>METESGNQEKVMEEESTEKKKEVEKKKRSRVKQVLADIAKQVDFWFGDANLHKDRFLREQIEKSRDGYVDISLLVSFNKMKKLTTDGKLIARALRSSAVVELDLEGTRIRRKKPLGERPKDEDERTVYVELLPKNVNHSWIERVFGKCGNVVYISIPHYKSTGDPKGFAFVEFETKEQAAKAIEFLNNPPEEAPRKPGIFPKTVKNKP[2x]

LARP7 is the family member showing the highest sequence similarity to La, with the characteristic La module in the N-terminal third of the protein. However, while La binds all nascent transcripts synthesized by RNA polymerase III via their shared termination motif, UUUOH, LARP7 binds almost exclusively to the non-coding RNA 7SK. The 7SK-specific 5′ cap is mono-methylated at the gamma phosphate of the 5′ triphosphate by another component of the 7SKsnRNP, MePCE (also called BCDIN3 in Drosophila). Together, MePCE and LARP7 bind 7SK on both ends, thus forming a stable 7SKsnRNP core protecting the RNA from exonucleases. Following a short unfolded region containing positively charged amino acids (1–27), the La module comprises two structured domains, one containing the LAM (residues 28–111) and the second, an RNA-recognition motif (RRM1; residues 120–199) according to a global analysis of the LARP superfamily.

The crystal structure of the LARP7 N-terminal domain, described here, is the first 3D structure of the La module of a member of the LARP family different from La showing the linked domains of the La module in a complex with RNA. The structure was solved from a crystal obtained in a drop initially set up with the hairpin HP4 (300–332). Indeed, difference Fourier showed densities for only three and five nucleotides in monomers A and B, respectively. The triplet of uridines at the 3′-end of 7SK binds into the cleft between the LAM and RRM1 domains. It is constrained in a characteristic hooked conformation, allowing strict recognition of the penultimate uridine, with a contribution of the RRM1 revealing LARP7 specificity. As was observed in La protein, the penultimate U-2 (numbering as in La) is anchored at the bottom of the crevice, and U-1 (the 3′-terminal uridine) at the surface of the LAM domain. The uridine U-3 stacks on U-1, leading to a characteristic fishhook shape of the backbone. The base ring is sandwiched between Phe44 from LAM and His138 from RRM1, in a pocket closed by Tyr153 from RRM1. Interestingly, the present crystal structure of the human LARP7 shows RRM1 to be smaller than the standard fold, with a β-sheet of only three strands. There is no additional C-terminal helix (α3 in HsLa), but helix α2 is one turn longer than in La, and extends to the last visible residue, Asn188.>GAMASHKLLVTPPKALLKPLSIPNQLLLGPGPSNLPPRIMAAGGLQMIGSMSKDMYQIMDEIKEGIQYVFQTRNPLTLVISGSGHCALEAALVNVLEPGDSFLVGANGIWGQRAVDIGERIGARVHPMTKDPGGHYTLQEVEEGLAQHKPVLLFLTHGESSTGVLQPLDGFGELCHRYKCLLLVDSVAFLGGTPLYMDRQGIDILYSGSQKALNAPPGTSLISFSDKAKKKMYSRKTKPFSFYLDIKWLANFWGCDD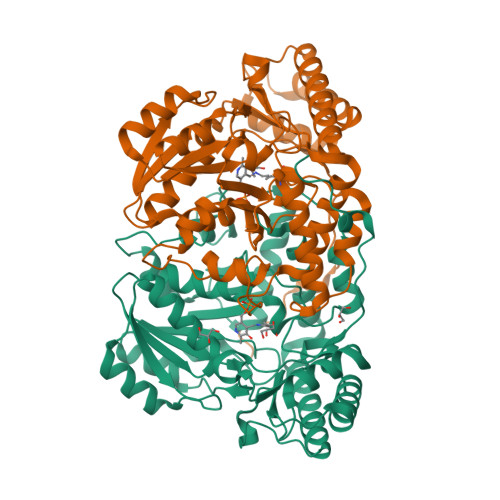QPRMYHHTIPVISLYSLRESLALIAEQGLENSWRQHREAAAYLHGRLQALGLQLFVKDPALRLPTVTTVAVPAGYDWRDIVSYVIDHFDIEIMGGLGPSTGKVLRIGLLGCNATRENVDRVTEALRAALQHCPKKKL[4x]The TRAPP complexes are nucleotide exchange factors that play essential roles in membrane traffic and autophagy. TRAPPII activates Rab11, and TRAPPIII activates Rab1, with the two complexes sharing a core of small subunits that affect nucleotide exchange but being distinguished by specific large subunits that are essential for activity in vivo. We report a cryo‐EM structure of the entire Drosophila TRAPPIII complex. The TRAPPIII‐specific subunits TRAPPC8 and TRAPPC11 hold the catalytic core like a pair of tongs, with TRAPPC12 and TRAPPC13 positioned at the joint between them.

To assign the eight small subunits within the core, we used the crystal structures that have been obtained for several of these subunits from mammals, either singly or in subcomplexes comprising up to four subunits. These were used to model the seven Drosophila core subunits which were then built into the density map. The subunits could be readily fitted into the map with the assembly of all seven, with TRAPPC3 being present twice, creating an octamer that forms the central flattened rod (and EV3). As expected, TRAPPC1 and TRAPPC4, which form the catalytic site to activate Rab1, are at the centre of the rod, flanked on either side by a TRAPPC3 subunit (C3a and C3b). TRAPPC1 and TRAPPC4 share a longin domain fold, with TRAPPC4 also having a PDZ‐like domain that protrudes from one side. The absence of this domain in TRAPPC1 leaves a groove on the other side of the rod, which is partially occupied by the C‐terminal region of one of the two TRAPPC3 subunits (C3b). TRAPPC5 and TRAPPC2 bind one TRAPPC3 (C3b), and TRAPPC6 and TRAPPC2L bind the other (C3a). TRAPPC1, TRAPPC5 and TRAPPC2 are known to be related to TRAPPC4, TRAPPC6 and TRAPPC2L, respectively, and so the octamer has an approximate two‐fold rotational symmetry, suggesting that it evolved by gene duplications adding, or altering, one half. In the octameric assembly, the greatest divergence is between TRAPPC5 and TRAPPC6. TRAPPC5 contains a disordered N‐terminal region and an extra C‐terminal α‐helix that is not present in TRAPPC6 (Fig EV3).

>[2x]MSRQASRLDAKKVNSEFLTLTYGALVTQMLRDFENAEDVNKQLERIGYNMGMRLIEDFLARTSAPRCLEMRETADRIQQAFRIYLNIQPTISNWSPASDEFSLVFDSNPLTEFVELPPDLTNLRYSAILSGCIRGALEMVQLEVQCWFVQDQLKGDNVTELRVKFVRRLEEVIPAGEDLEVLFQGPVASWSHPQFEKGAV;> MSEEILFDCLHAEIVNYCLDSNKEHDLATLEYIGFTTGYRLIERLTREVSRFKDELETMKFICTDFWMLIYKKQVDNLRTNNHGMYVVQDKAFRFLTRISPGTKQLEHAPKFVAFTCGLVRGALSNLGINSTVTAEVQSIPACKFHIEVNRN;> MTIFNLYIFDKFGTLLHYAEWNRTKKSGITREEEAKLTYGMLFSIKSFVSKISPHDPKEGFLYYKTNRYALHYLETPSGLKFVLNTDTTAINVKELLQQLYAKVWVEFVVRDPLWTPGTVVTSELFQSKLDEFVRQSPIFGIRNI;> MIIYGVYIVSKSGGLIFNLDNNVPRIEHEKTFTYPLDLVLDYDSKKVSVSFNRKDGINVGHVLVAVNGMPVNGVTLDDGRDVRTTLDAPENYPINLKFSRPKMTTNEKIFLASMFYPLFAIASQLSPEPKSSGIEILEADTFTLHCFQTLTGIKFIIISETGLNGIDLLLRKVYELYSDYVLKNPFYSLEMPIRCELFDNKLQELLAQVEKTGISNIDK;> MSTYYFVIVGQNDNPIYEKEFSTVNKELRKEDHRHLTQFIAHAALDLVDEHKWKTANMQLKSIDRFNQWFVSAFITASQIRFIIVHDNKNDEGIKNFFNEMYDTYIKNSMNAFYRINTPIKSPMFEKKSEIFGRKYLLS;> MEKLEALKISSMRPRSNILDRPLSKGKTEVSQSIVALLFSEIVQYSQSRVFTVPELQTRLHDLGQDVGTRIIDLYFVRERSSKRETKLTQMLLFVKTTVWKNLFGKEAEKLEHANDDERTYYIIEKEPLVNTFISVPKDKGSLNCANFTAGIVEAVLTNCGFPCKVTAHWHKGTTYMVKFEDFVIARDKQMEEK;> MAFCIAVIGKDNAPLYLTTSDMEQELELQYHVNAALDVVEEKCLIGKGAPESKELYLGLLYSTENHKIYGFVTNTRVKFIVVIDSSNVALRENEVRAIFRNLHLLYTDAICNPFYIPGESLTSKKFDRAVQKLMSGTA>[4x]MSVIKSDMKIKLRMEGTVNGHKFVIEGEGEGKPYEGTQTMNLKVKEGAPLPFAYDILTTAFHYGNRVFTKYPKDIPDYFKQSFPEGYSWERSMTFEDGGICTATSDI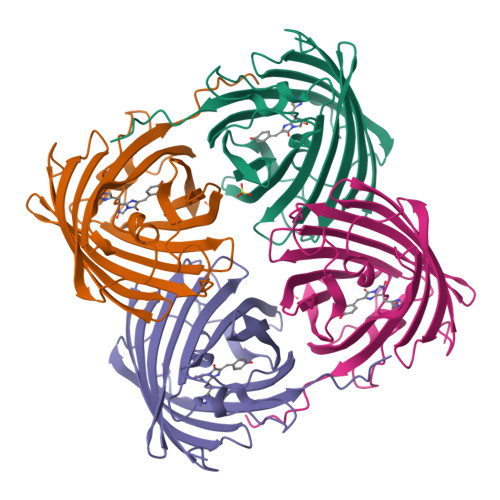TLEGDCFFYEIRFDGVNFPPNGPVMQKKTLKWEPSTEKMYVRDGVLMGDVNMALLLEGGGHYRCDFKTTYKAKKGVQLPDYHFVDHRIEILSHDKDYNNVKLYEHAVARYSMLPRQAKHHHHHH> TGYVGLKNQGATCYMNSLLQTLFFTNQLRKAVYMMPTEGDDSSKSVPLALQRVFYELQHSDKPVGTKKLTKSFGWETLDSFMQHDVQELCRVLLDNVENKMKGTCVEGTIPKLF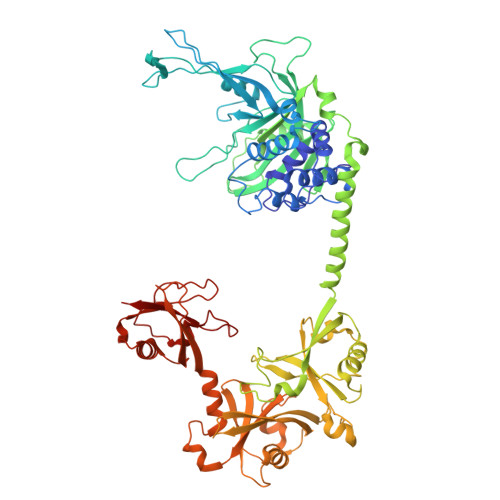RGKMVSYIQCKEVDYRSDRREDYYDIQLSIKGKKNIFESFVDYVAVEQLDGDNKYDAGEHGLQEAEKGVKFLTLPPVLHLQLMRFMYDPQTDQNIKINDRFEFPEQLPLDEFLQKTDPKDPANYILHAVLVHSGDNHGGHYVVYLNPKGDGKWCKFDDDVVSRCTKEEAIEHNYGGHDDDLSVRHCTNAYMLVYIRESKLSEVLQAVTDHDIPQQLVERLQEEKRIEAQKRKERQEAHLYMQVQIVAEDQFCGHQGNDMYDEEKVKYTVFKVLKNSSLAEFVQSLSQTMGFPQDQIRLWPMQARSNGTKRPAMLDNEADGNKTMIELSDNENPWTIFLETVDPELAASGATLPKFDKDHDVMLFLKMYDPKTRSLNYCGHIYTPISCKIRDLLPVMCDRAGFIQDTSLILYEEVKPNLTERIQDYDVSLDKALDELMDGDIIVFQKDDPENDNSELPTAKEYFRDLYHRVDVIFCDKTIPNDPGFVVTLSNRMNYFQVAKTVAQRLNTDPMLLQFFKSQGYRDGPGNPLRHNYEGTLRDLLQFFKPRQPKKLYYQQL>[3x]MNSQLTLRALERGDLRFIHNLNKELARYE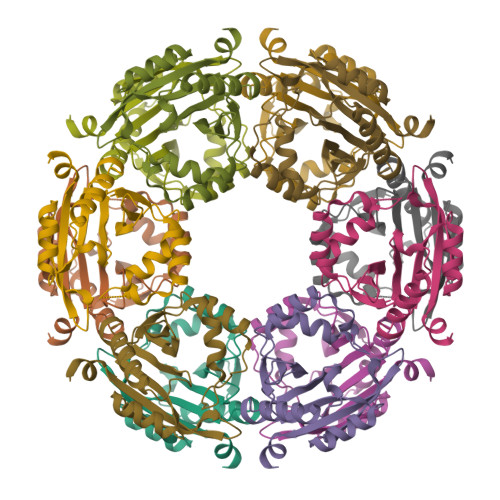YMEEQPYESFDELEELYNKHIHDNAERRFVVEDAQKNLIGLVELIEINYIHRSAEFQIIIAPEHQGKGFARTLINRALDYSFTILNLHKIYLHVAVENPKAVHLYEECGFVEEGHLVEEFFINGRYQDVKRMYILQSKYLNRSE> MRRAVVSSSPPPSYESVMAQATLEVPFVPPRYMAPTEGRNSIRYSELAPQYDTTRVYLVDNKSADIASLNYQNDHSNFLTTVVQNNDFTPAEASTQTINFDERSRWGGDLKTILHTNMPNVNEYMFTSKFKARVMVARKHPEGVVETDLSQDKLEYE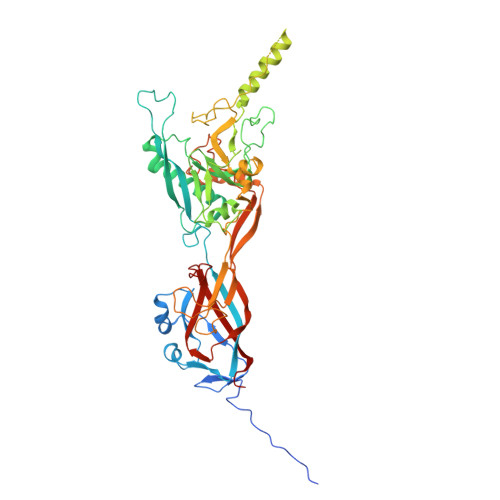WFEFTLPEGNFSETMTIDLMNNAILENYLQVGRQNGVLESDIGVKFDSRNFKLGWDPVTKLVMPGVYTYEAFHPDVVLLPGCGVDFTESRLSNLLGIRKKQPFQEGFRIMYEDLEGGNIPALLDVPKYLESKKKVEDETKNAAAATADTTTRGDTFATPAQETAADKKVEVLPIEKDESGRSYNLIQGTHDTLYRSWYLSYTYGDPEKGVQSWTLLTTPDVTCGAEQVYWSLPDLMQDPVTFRSTQQVSNYPVVGAELMPFRAKSFYNDLAVYSQLIRSYTSLTHVFNRFPDNQILCRPPAPTITTVSENVPALTDHGTLPLRSSIRGVQRVTVTDARRRTCPYVYKALGIVAPRVLSSRTF> AGVGTVPMTDYGNDIEYYGQVTIGTPGKKFNLDFDTGSSDLWIASTLCTNCGSGQTKYDPNQSSTYQADGRTWSI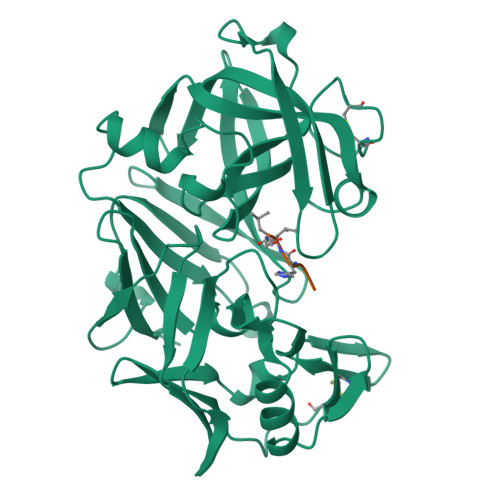SYGDGSSASGILAKDNVNLGGLLIKGQTIELAKREAASFASGPNDGLLGLGFDTITTVRGVKTPMDNLISQGLISRPIFGVYLGKAKNGGGGEYIFGGYDSTKFKGSLTTVPIDNSRGWWGITVDRATVGTSTVASSFDGILDTGTTLLILPNNIAASVARAYGASDNGDGTYTISCDTSAFKPLVFSINGASFQVSPDSLVFEEFQGQCIAGFGYGNWGFAIIGDTFLKNNYVVFNQGVPEVQIAPVAE>GMYGKGKSNSSAVPSDSQAREKLALYVYEYLLHVGAQKSAQTFLSEIRWEKNITLGEPPGFLHSWWCVFWDLYCAAPERRETCEHSSEAKAFHDY[2x];> GGIGRHTPYGNQTDYRIFELNKRLQNWTEECDNLWWDAFTTEFFEDDAMLTITFCLEDGPKRYTIGRTLIPRYFRSIFEGGATELYYVLKHPKEAFHSNFVSLDCDQGSMVTQHGKPMFTQVCVEGRLYLEFMFDDMMRIKTWHFSIRQHRELIPRSILAMHAQDPQMLDQLSKNITRCGLSNSTLNYLRLCVILEPM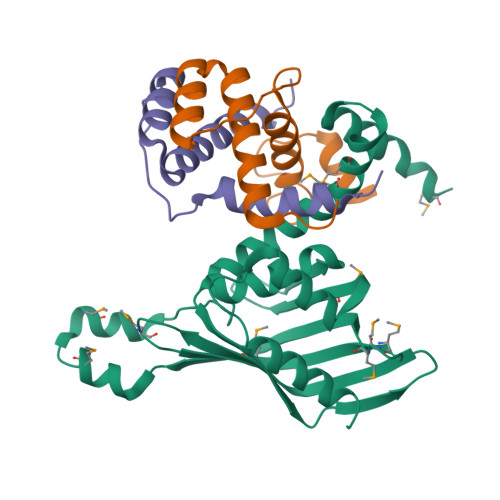QELMSRHKTYSLSPRDCLKTCLFQKWQRMVAPP>[4x]MSNCQYKIYPPLGIARVGNGPAIKPLSLSTPEVPWAHLYDTNVQYLVTQQELEQLLEEAFGGNVINEISQIKTKLDERKAE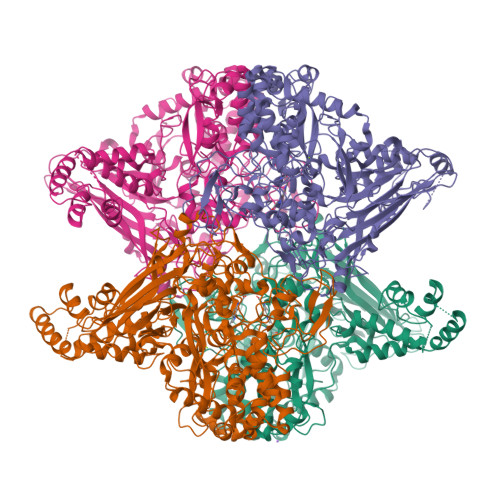KFKQEEIETITGLLGLSHLVPQQQLSRSLDNLELKSTKDSDDIVQQIKGALLKVLSDHYLHAVKKQAQNFYIYKCDEQGNPVEKLKLTDGDKVTWRVEVANKKSFWYDYNNALDLSLHTQGSGNLSKNVSKHRLAPAMTAKRRNPNVITNSLRKQLVISSQGSVSSDNNTQVPLRGKFPANEPDTNNRLSDLLNLQERHNVLQGSIECDNEGVLRFYAGNGISQALSPSSLNTDFADNSNWFDDICDGRVTAVVELKNGDTFEIQDEQSSAWVATTPPDYAPQIEPIVTMYDMVSGAALKEQDLDNLTTQFSDVFPILYRLYRMQWVNQADFTDNAVNTQIRELNSELGFAQLLDNSASAKSLREGIFNQFRNPLFDQDIDVDDPGQSSNEWVSNSRIIPSKDETNIAAKPATSSLKLPFYPNDGIDYPGSPVQWFAIPPFMYQHLQNWAAGDFSVTQVEKESANTIEELGLFYSEQFKNSPNSALLCARGALDALYGGGFHPGVELTWPMRHNLIYSQNDYVSSVTPEINLLGLREFRLKQDLQGLNSPNMYQDFGHVIAVDNVTASIDPNSDAAWLWRSTPGDLTKWMGIPWQSEAASCQAVYTPEDFPIPSWXAANLPVHVLPLARYNKFKDSQSADLPEINGMTHSIAQGMSEETFEHLRLEQFSQRLDWLHTADLGFVGYHAEGGYTNGLIQMVSQWKNMAMVMARPVENPGSSGIPNVVYVAYSQADKD> ELQSPEYKLSKLRTSTIMTDYNPNYCFAGKTSSISDLKEVPRKNITLIRGLGHGAFGEVYEGQVSGMPNDPSPLQVAVKTLPEVCSEQDELDFLMEALIISKFNHQNIVRCIGVSLQSLPRFILLELMAGGDLKSFLRETRPRPSQPSSLAMLDLLHVARDIACGCQYLEENHFIHRDIAARNCLLTCPGPGRVAKIGDFGMARDIYRAGYYRKGGCAMLPVKWMPPEAFMEGIFTSKTDTWSFGVLLWEIFSLGYMPYPSKSNQEVLEFVTSGGRMDPPKNCPGPVYRIMTQCWQHQPEDRPNFAIIL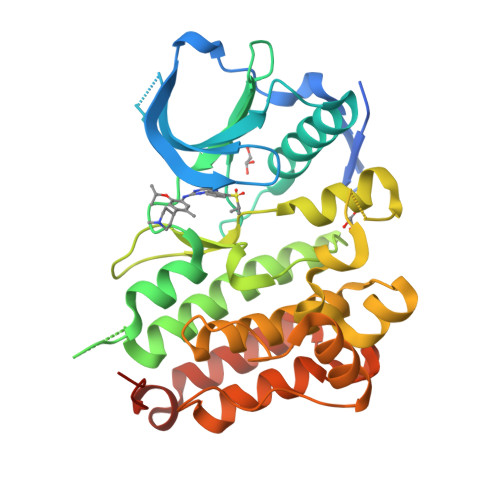ERIEYCTQDPDVINTALPIEYGPLVEEEEK>SMVEYTKESVQADPENWRSVDPDNLVIFETTKGVVYIELAPEIAPNHVAQIRKVVRTGLYSGTKFHRVISGFMAQGGDIAATLGREPDLEAVDGEFVFRRDPKSIVLTVINEEDQTKSQYTGFYNGFPIETRQDELANYSEDKRVESWMPHCAGVVSMARTNDPNSGKDQFFLMRDESRFLDRKYSSWGRMLEGLDVAKSLTIGEPPERPDILVSAVMVSDLAPKDRPEAWVMRNDGPMFSLFLDRMGRDKDVCSLPQTPSVVFVSEDKEG[2x]

Hirschia baltica contains two cytosolic and five periplasmic canonical single-domain PPIases, but also two large, homologous cyclophilins with 293 and 300 residues, which we term AquaCyp293 and AquaCyp300, respectively. Our data reveal a unique two-domain architecture of AquaCyp proteins, in which the catalytically active cyclophilin domain maintains extensive contacts with a composite domain formed by terminal extensions and internal insertion elements. The crystal structures of AquaCyp293 and AquaCyp300 demonstrate that AquaCyps fold into two domains, a classical cyclophilin-type PPIase domain and the NIC domain with a novel mixed alpha-helical/beta-strand structure. Both AquaCyp proteins are stabilized by a conserved inter-domain disulfide bond.

AquaCyp293 is a monomeric protein based on size exclusion chromatography—multi angle light scattering (SEC-MALS). AquaCyp293 is a highly active PPIase. Similar to the highly active human Cyp18, AquaCyp293 shows very high kcat/KM values, which range between 106 and 107 M-1s-1, and the maximal differences between peptides are only 6-fold (between Leu-Pro and Glu-Pro). AquaCyp293 thus resembles other cyclophilins in both high PPIase activity and low substrate specificity. With a kcat/KM value of 1.0 × 104 M-1 s-1, AquaCyp293 catalyzes prolyl isomerization in a folding protein about 100-fold less efficiently than in the tetrapeptide substrates. Most of the residues known to be important for activity in hCyp18 and EcCypB are also conserved in AquaCyp293, in agreement with their catalytic competence. The residues Arg65 and Gln73 of AquaCyp293 correspond to Arg55 and Gln63 in hCyp18 and are essential for catalysis. The C-terminal extension forms an elongated structure that contacts the N-terminal extension, the inserted domain, and the cyclophilin (PPIase) domain. It starts with two short 310 helices and continues into β-strands, which provide a structural link with the β-strand of the N-terminal extension and a β-strand (Ser259-Phe262) of the cyclophilin domain.>[2x]MAPVPEPEVVATPPADAGRGLIRVDSREIRHYSGTRKEPDYLVSRDNGKTWEMKAAPAGYPPNYGGIPKESPAIVRNPLTREFIRVQPIGGFVFLSRGGLDGKWLAVTNDGKLEEDWKDPEKRKNLKKLGGIMRTPVFVNKGRRVIVPFHNMGGGTKFHISDDGGLTWHVSRNGVTSPRHEARPPHQGVRWFNNAVEATVLEMKDGTLWALARTSQDQAWQAFSKDYGETWSKPEPSRFFGTLTMNTLGRLDDGTIVSLWTNTMALPENATAGNGTWEDVFTNRDSHHIAMSGDEGKTWYGFREIILDEHRNHPGYATLDGPEDRGKHQSEMVQLDKNR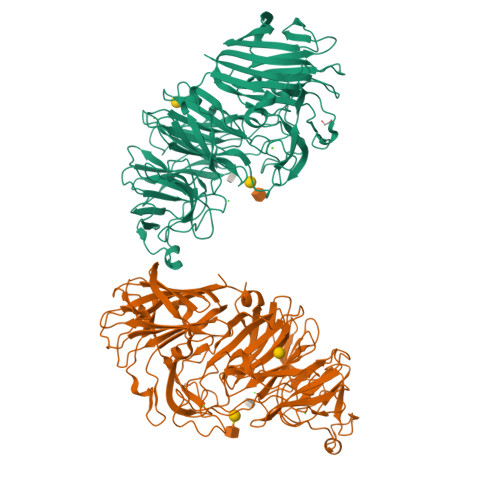ILISLGQHKNHRRLVIVDRRWVGAKTRATQTGKDLDSQWTIHTYIPQKKGHCSYNRKPSAELVQDPSGGTKKVLQIKRLDDPELVNEKSNVDYRNGGATWNFPNGTTGLVKFRFRVVDGEQADDSGLQVSLTDRLFNACDSTTKDYALFTFPIRLKPAPHLLLGMKKVPFTPGAWHEISLLWQGGQAVVSLDGKKAGTLKMANKSPNGASYIHFISTGSQPDAGILLDTVNARVKLE>[2x]MGSDK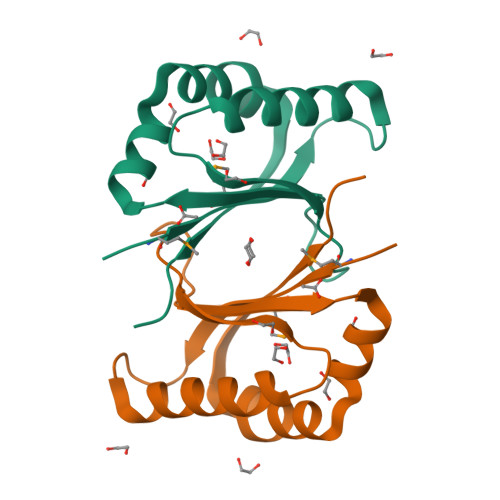IHHHHHHENLYFQGMIRHTVVFTLKHASHSLEEKRFLVDAKKILSAIRGVTHFEQLRQISPKIDYHFGFSMEFADQAAYTRYNDHPDHVAFVRDRWVPEVEKFLEIDYVPLGSVV>[3x]MHYAEAATPAKSAGSAVAKKHLEAKQKIGFVHGIDGTIATIAPAASKVTVPYNTVLEIAVSATNIANALVFNLEKDGSIGVILLDNISEVRSGQDVYATGSLLKIPVGFHMLGKIINPLGKEIPTGLFTKAAPLLDDTKLGLVEEMAPNIVSRQPVNYNLLTGYKVIDTLIPVGRGQRELILGDRQTGKTSIALSTILNQTKVNNEILSKNNVLSVYVSIGQRCSNVARIHRLLTEYDAMKYCTIVAATAADPAGLQYLAPYAGTTLGEEFRNSGRHILLVYDDLSKQAVSYRQISLLLRRPPGREAYPGDVFYLHSRLLERSAMMSPQKGSGSLTSLPIVETLSNDVTAYIVTNVISITDGQIYLDAKLFTGGQRPAVNIGLSVSRVGSSAQNKAMKKVGGALKMLMGEYRKMAGEQTSGSQNVSPVMIRGARCLQLFNQKGPSYFMDAIVALYAVTNGYMDDVKLQYSKFYEFLLLNKDLPVLYGQVNNKYFYMYNKNLNYFIRYFGLNHEILEPELKKYIEIHTNLFLDNYQSRMNELKSDEDLVQLKNLLYACKRTV;>[3x]TAPATAADVKQVGYVQQIIGAVVDVTFTDSVPPVLTALTVDAKETGTLLTMEIVQHLDTKTARCICMSSTDMLRLRTPVVNTGSQITVPVGEATLGRIFNVMGDAIDQRGPVKNKVRWPIHRKAPTLAEQSGKDEVLVTGIKVIDLILPYCKGGKIGLFGGAGVGKTVIIMELINNVAKGHGGYSVFAGVGERTREGTDLYLEMMGSKVIDLQGDSKCVLVYGQMNEPPGARARVAQTALTMAEYFRDEAGQDVLLFVDNVFRFTQANSEVSALLGRIPAAVGYQPTLAEDLGMLQERITSTVKGSITSVQAVYVPADDITDPAP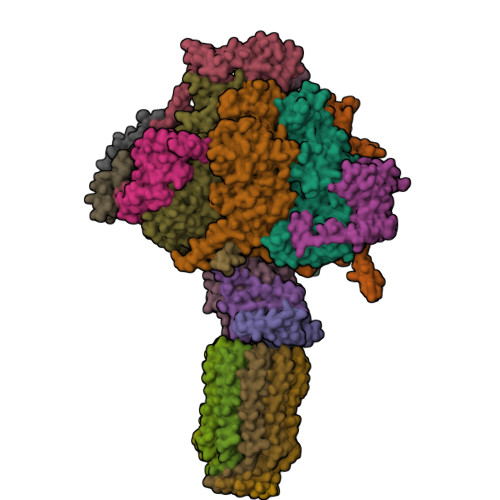ATTFSHLDATTVLSRSVAEAGIYPAVEPLECASRIMDPDAIDVNHYNVAMDIVEMLTKYKELQDIIAVLGIDELSEEDKLIVDRARKVAKFMSQPFAVAEVFTGMKGYYVQLEDCVSDFGSLLMGQCDNIPEMAFYMVGGLDSVKEKAAKMAAEAAAMRERARKAAEAK;> MPGGGTIRFWREKLEGYKKYHQIVKTIKMVTLAKYRQTVVRTRVRDQTLRYTRKALDAKTQDDQEVIEKSECLLYVPITTNRGSCGALNTNMVRYLQEVENPKMTIISVGKKALDAMTKVFQDTYRRTILNDMKQAMSFQFAAYVLEHMNTVPWDRAQIVYNRYHGAASQKLAIFNLPKFEDWKQKLEEDSAGDGKIEEDGLLQSLPMKTALGELEETAVEDFYNFHSCLAVLNAVSENELSEYAARIVAVENQLGNITGLMQLADYTYNKTRKELITAELLEIIGTMTAMHAGKKVGLKKTEFWK;> MRASRTLLLSVSRFMRQDPRKFFPDNGFRFFDGPEDSFGDGNIPAQIILTLTRQDEFILKQEPVAAITIRTNEGEMGVLAGHEYTVQQLAPGILEVEYEGGKKDQYVISGGFAHVNDTGVVDINTVEAVPLEEIDHEKLAKALEEARAKSQSPDEAVRIQGEIALEIFEPLEAALH;> MSWRDAGISYLRYLSIVTRCIHEVQKEGPLLTKNVRFSTIGWKSLYLDHGATKEYTAIPAELEKIPENQVAQQHHA;>MQKLSRVVCNRLVRFHGTVAASAGGKRYDLFGYEVSVATGPFIEEIKKAQFYDDAGEVIVKMNLANTPPDLQTYNAVLERILNCKSKRSQPVKGENKFAAMMDILEEMDARSGIKPNAESWGYVLKELVQAGDFRLGWVCIAGMKSLGITPDQALVDANEANAAKAKAAGTDFPAYLKKAAPESFDTKAWGI[3x];> MHMRRAVSVFGRCRSLNGLRNYAVPSPKYIEIYQSDFSRNAYPLELLGGSHVDFAKLLYSFADQVENKKFEVYVEDFKKLDSIIAEKGPFWAEEKIFQSPTFQGLSEGFKFILGWIQSEGAIDRLENVRLAYKELVNEARKETTATVIVAKEPSGNDLAEIRKQVEELHKESPLKDYKLVLETKVDPSIGGGYILEVCNQVVNRSAAAAAAETAALAKASAAQVDWTSLPAAPPRPSPSAPDTLIRLLGSVVDDLADADKVEQKYGA;> MAAACAVRGFTTARPMLTPNKVKVPGRKPQDEEDLTWAEADRKLTPEERYARDKQMALLDKMTSQVEELEKSHTEQKKSNKGVKAQIEAISRQLEALKAQLKE;>MQRGSSITKVVRRAALARSTRNAAIAYEVTVNGANLIGAGMAASGVGVPAIGVAMCFSSYMLAAARQPNMSAKLLPYCILGFALSEALALFTLLIALLELFVFS[10x];> MFRGFRPVLAADAVKFQTLYNVLTGKQHLKDQVPVKDCNLTAIFGASWKADLNKWFDSEYAPKLPAAERDSAKKSLDLYLKRVDLTRYTREELTTYGILACGPGKVDALTEKHLLETGKARLEELTAGLGNKDEGVNAFRKEVEQEGKYANWPAEKSKALADKVIAASP;> MMRRACRIIRPSHVRGVSGVAPTIYLRSKAALPATSTTDVRPQLYALQRFAKAQLKTATEAERAAIEADIARYQEYLDSDLEKLKQDVAEDTAKKQKLIPLLDRYPDVPIEKIPEHANVLLKKIDACLEILSKDIGEVTDAEAHEMYFETSKFQILHIYTGCVASFPEGDVPPGAVECLPGQVIRTKVNGEDVMLEIDEVDPGYQVCWFKPDVPLPENAEILWSYPYEPTAALPTGTTWEEGQANVLIPAEPTPEAAVWPPTPVTNVYAPMAEKLALKSNPELKVLFKEALLQPAKLLPLDVDYQCSHDREVVEAKRDRYLTALVEAEQAPPLPFTPDVLQLQLEHNVLKGELIDRLRALEYTIVTEQLQARLHERRLRGDVIDEWEELDYHPLVRDDTYLAIDFGDPTFGRYIWKLFPHTDGDEECMFKDTRLDVLPPQVNPLNAILAQHTAQTPVHRSLEKRLWTEVRATAVSE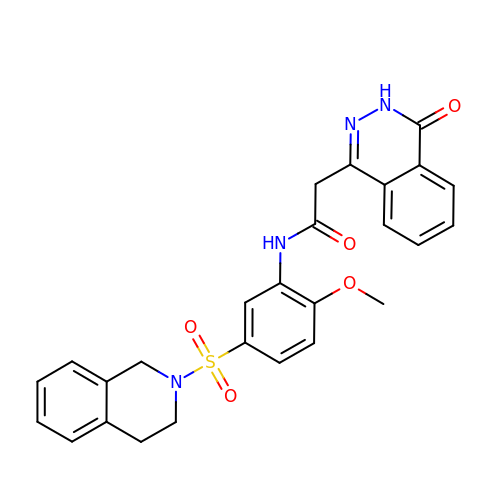~{N}-[5-(3,4-dihydro-1~{H}-isoquinolin-2-ylsulfonyl)-2-methoxy-phenyl]-2-(4-oxidanylidene-3~{H}-phthalazin-1-yl)ethanamide | C26 H24 N4 O5 S | OBCUZJPWFQZKTN-UHFFFAOYSA-N> YDGTNCKAPGNCWEPKPD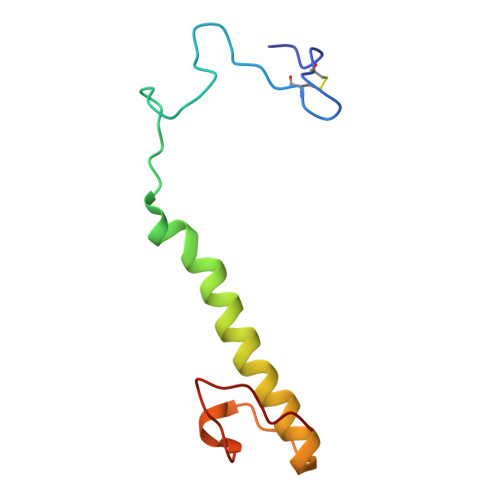YPAKVEGSKYDPQHDPAELSKQGESLAVMDARNEWRVWNMKKTGKFEYDVKKIDGYDETKAPPAE>ERIIQQTDYDALSCKLAAISVGYLPSSGLQ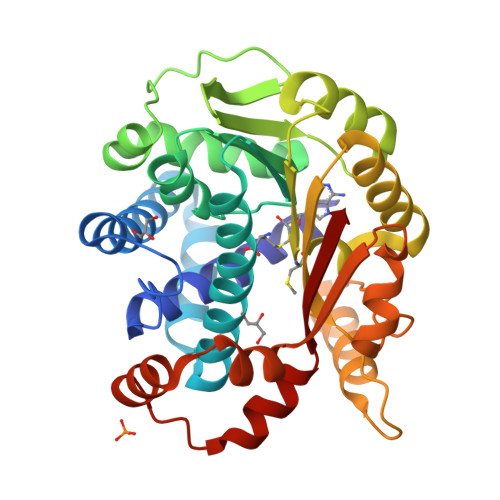RLSVDLSKKYTEWHRSYLITLKKFSRRAFGKVDKAMRSSFPVMNYGTYLRTVGIDAAILEFLVANEKVQVVNLGCGSDLRMLPLLQMFPHLAYVDIDYNESVELKNSILRESEILRISLGLSKEDTAKSPFLIDQGRYKLAACDLNDITETTRLLDVCTKREIPTIVISECLLCYMHNNESQLLINTIMSKFSHGLWISYDPIGGSQPNDRFGAIMQSNLKESRNLEMPTLMTYNSKEKYASRWSAAPNVIVNDMWEIFNAQIPESERKRLRSLQFLDELEELKVMQTHYILMKAQW[3x]formyl phosphate | C H3 O5 P | 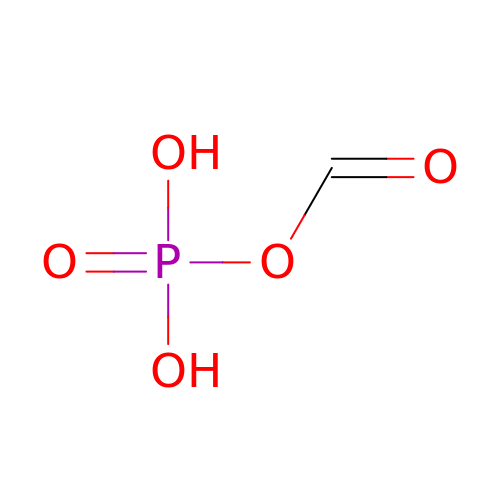TVISEJUYYBUVNV-UHFFFAOYSA-N>[2x]SGWRAPSCTKV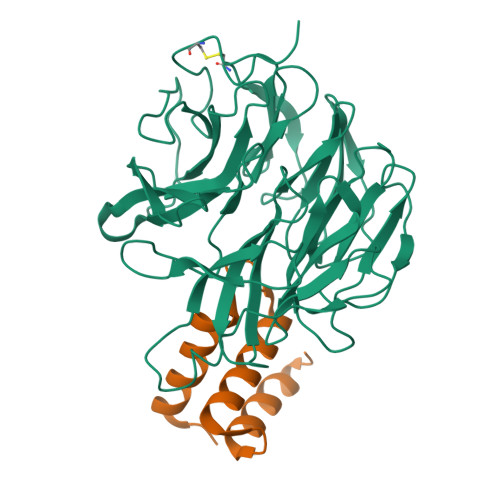TGDGAVTFTTDDGATLAPTTGTLQSVSYTHGLVALDTPNTLLATHNDELQRSTDAGCTWTKVATLGSGSTWLTAATGGRAFAWEKNGGYLARVDGRTVTKLSSPSADIVGVGTDKARRDHVRLAGSDGQLYDSTDAGATWKPLGKLAFGPGASVYTVSFDPADLDHAVAGGMTTGGAVTTDGGATWTAATGLSATAGGKSNLFAASVSPADRNVVYALGIDLVEAAPNSGAEGRHLYRSTDGGRTYTRIVDDTPDTELTNSTLLAPSPVDPNVLYFEYGTYFQAYGTDLYRYDARTGKVGKTHNAHDGISAIAFNPARPSVMYLGLEEVQI;>[2x]VVGIGRDKLGKIFYRALTQYLTPTSNFSQLRAAAVQSATDLYGSTSQEVASVKQAFDAVGVK>[2x]DNILYSGETLSTGEFLNYGSFVFIMQEDCNLV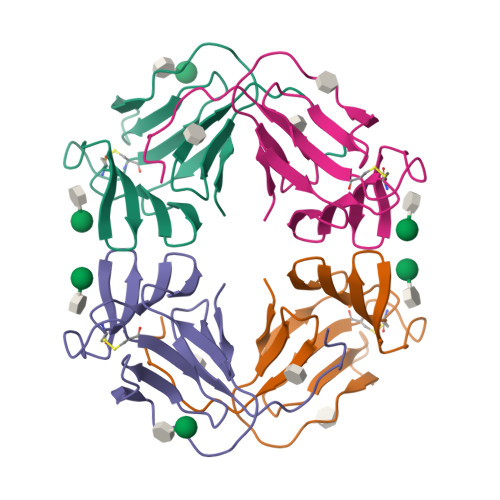LYDVDKPIWATNTGGLSRSCFLSMQTDGNLVVYNPSNKPIWASNTGGQNGNYVCILQKDRNVVIYGTDRWATGTHTG> MVMAVNLHKHQKNLVYRLSQQYLAAARDLAADVRSEKQLQQYYTLVRQCVHGLRYVKDGFQLTVEEDIQVTLQLARVLLEETHEVELAEQYLGSLRTRLRTTPLTDARHAVEFQLLYDVPLAKEDRAELRQVVRHTTGLLEELADSDAWAWLFRYCRIIGLEAGGARSNSAVLQEYLKLLQLVSAGPVGLHAFVLCSCVAFILDRVVELDRSLLTQLRALRKAGTAIPLQLQMWSLLLDLLVAIQLDENIMDLLTDFKDFFSTHKDALKDGDDTVVLSIKEGVNVRLFVPLFNYHDCKNILLLFQSVSYLTTCYSKSSNFSTKFLPKVLKTSQELKETLQKRTSLVHVQSIRNIYDKVVDLCRFYQTWESLILSERVEGGIPRLQYSEYNILLEAISSQQAQQADLSHVGRLYSTLTKSKDPELRLIGIAHLYTLIVAELSSCSEGPEGISELTQKTTDAWEQLQHAYLSSSLVQNNVWKCSVAILWAISRFEPFSGHPIHSSSNDQQTLYMQQLNEFFTDNALVGTPEAVPAKDFKLKKSLLLHFLLNYLGGTMLVSDVQKRCDISSSCFQMGKQQYMPGMRYVAGIWHLMNSTVAMKTKEV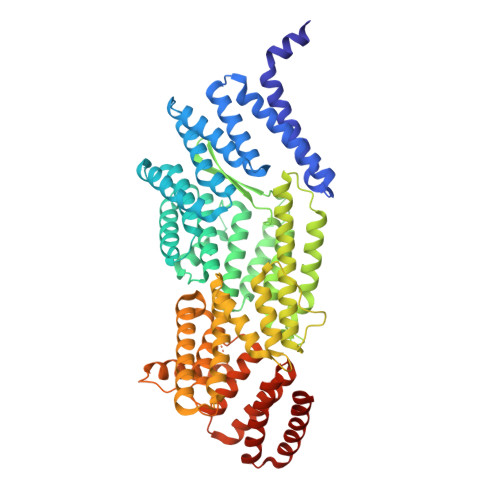AITRAKLEGLVDKMLNS> GGCUUAUCA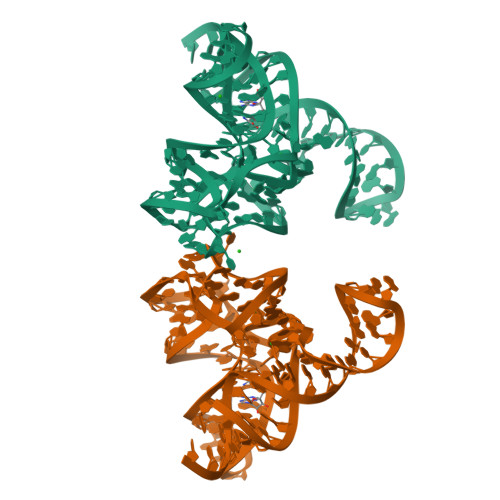AGAGAGGUUUAGGGACUGGCCCGACGAAACCCGGCAACCAGAAAUGGUGCCAAUUCCUGCAGCGGAAACGUUGAAAGAUGAGCCG>GTKYNSSPRDNFEALWRIMDENYCFFAFKDVDWDDVYDRYNLLVKDTMNQYELFDILGKMLAEVKDGHTNLISSFDMSRYWAWYEDYPANFYKEIQDNYLGTDYKIAGGMKYKRLADDQIGYVYYGSFSSGVGENNLDYMFAHFKECKGLIFDVRDNGGGSMLYSDRIASRFLEERILTGYTQYKKGNGHND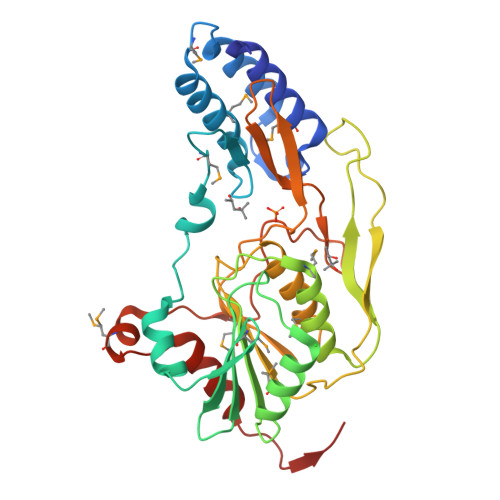FTQPNPVYLSPSDRTRWLRPVIVLTNRHSYSATNDFVNVMRLLPQVTVMGDRTGGGSGLPFSSELPNGWSVRFSACPVLDVNKQHTEFGIDPDTAVAITGEDIMKGRDTIIEAAIGLLLAKGDSAISY[4x]>[2x]MGSSHHHHHHSSGLVPRGSHMGYSATAPVNLTRPATVPSMDGWTDGTGAWTLGEGTRVV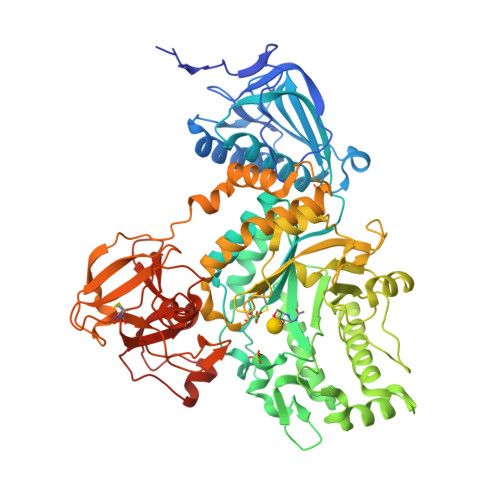SSDALAARAQSLASELTKFTDVDIKAATGSATGKDISLTLDASKKAELGDEGFKLNIGSKGLEVIGATDIGVFYGTRSVSQMLRQGQLTLPAGTVATKPKYKERGATLCACQINISTDWIDRFLSDMADLRLNYVLLEMKLKPEEDNTKKAATWSYYTRDDVKKFVKKANNYGIDVIPEINSPGHMNVWLENYPEYQLADNSGRKDPNKLDISNPEAVKFYKTLIDEYDGVFTTKYWHMGADEYMIGTSFDNYSKLKTFAEKQYGAGATPNDAFTGFINDIDKYVKAKGKQLRIWNDGIVNTKNVSLNKDIVIEYWYGAGRKPQELVQDGYTLMNATQALYWSRSAQVYKVNAARLYNNNWNVGTFDGGRQIDKNYDKLTGAKVSIWPDSSYFQTENEVEKEIFDGMRFISQMTWSDSRPWATWNDMKADIDKIGYPLDIREYDYTPVDAGIYDIPQLKSISKGPWELITTPDGYYQMKDTVSGKCLALFTGSKHLDVVTQVGARPELRNCADVSVGQDQRNTANERNTQKWQIRADKDGKYTISPALTQQRLAIATGNEQNIDLETHRPAAGTVAQFPADLVSD Human bestrophin1 (hBest1) is a Ca2+-activated Cl− channel essential for Cl− transport in retinal pigment epithelium (RPE). Although the structure of hBest1 is still unsolved, two Best1 homolog structures, one from bacteria Klebsiella pneumoniae (KpBest) and the other from chicken (cBest1), have been previously reported. Overall, the channel is a pentameric assembly with a single ion-conducting pathway, which varies in diameter along its length and is constrained at two narrow points: a “neck” contributed by three residues (I62/I66/F70 in KpBest and I76/F80/F84 in hBest1/cBest1) on a transmembrane helix, and an “aperture” formed by a single residue (I180 in KpBest1, I205 in hBest1, and V205 in cBest1) on a cytosolic helix. Here, by electrophysiological and structural analyses, we show that the neck and aperture in hBest1 are both indispensable Ca2+-dependent gates, and their dysregulated opening by rationally designed or patient-derived mutations causes Ca2+-independent leak and elevates Ca2+-dependent channel activity.

A patient-derived mutation of hBest1 at the aperture, I205T, was previously reported. As threonine has a shorter side chain than isoleucine, we speculated that I205T, like I205A, enlarges the opening at the aperture and enables Ca2+-independent leak activity. Notably, the threonine side chain possesses a hydrophilic hydroxyl group that is capable of forming H-bonds, which can further affect ion permeation. To test this idea, we solved the crystal structure of the equivalent KpBest I180T mutant at 3.2 Å and examined hBest1 I205T in HEK293 cells by patch clamp. Remarkably, the aperture of KpBest I180T was dilated to a size (radius 2.1 Å) bigger than dehydrated Cl− but smaller than CH3SO3−, while hBest1 I205T conducted robust Cl− current but no CH3SO3− current in the absence of Ca2+. Moreover, hBest1 I205T showed a CH3SO3− to Cl− relative permeability similar to that of hBest1 I205A and retained CH3SO3−-mediated trans effect, reaffirming the critical roles of the aperture and the neck in ion selectivity and CH3SO3−-promoted channel opening, respectively. Therefore, our results indicate that hBest1 I205T is a gain-of-function mutation due to incomplete closure of the aperture. Interestingly, asymmetry of the aperture is observed in the KpBest D179A and I180T mutants, suggesting that “breathing”, which manifests as local, asymmetric changes in the aperture region, may additionally contribute to accommodate large ions, such as CH3SO3−. While mutants with conformational changes at the aperture (e.g., KpBest I180A, I180T) or neck (e.g., cBest1 3A) do not have structural alteration at the other restriction, a mutation near the aperture (D203A and D179A in hBest1 and KpBest, respectively) impacts both gates, suggesting both independent and cooperative regulations of the two channel gates.

>[5x]NAMIIRPEQHWFLRLFDWHGSVLSKIIFRLLLNVLMSIIAIISYQWYEQLGIHLTVAPFSLLGIAIAIFLGFRNSASYSRFVEARNLWGTVLIAERTLVRQLRNILPAEHDAHRRIVSYLVAFSWSLKHQLRKTDPTADLRRLLPEERVTEILASSMPTNRILLLAGNEIGQLREAGKLSDTTYGLMDNKLDELAHVLGGCERLATTPVPFAYTLILQRTVYLFCTLLPFALVGDLHYMTPFVSVFISYTFLSWDSLAEELEDPFGTAANDLPLNAMCNTIERNLLDMTGQHPLPE> 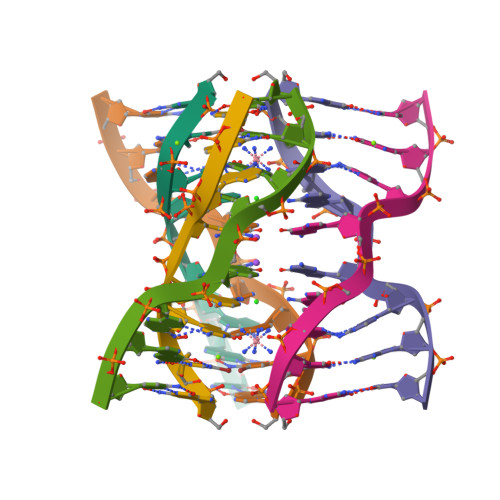GCGAGAGC> MQRCLARLFQAGVHTPHGSRYNAARMKNWPVQEVPQNFNFTNEQRFKAKAVPRDTGKIPRDFLLSVLYRNQPCEVASLWEHCLHDPQIVLDSKRHLREVLQQARAEGFVSFEKDAVTDRWVCHLTRERFEEVRALVGARAEAQDLYSGLRGASATETSAYSESFREMNEDTKREHFRLLSEQVADTTTHLRKFQ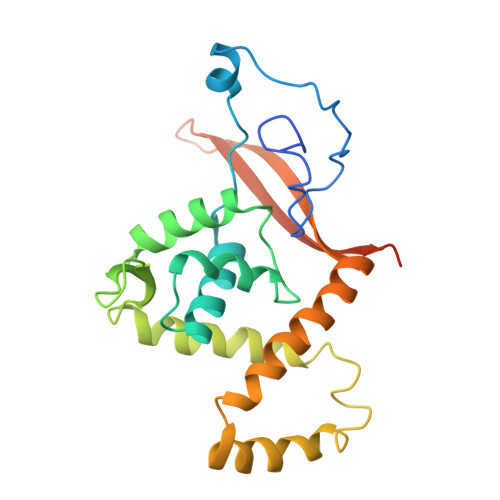RMEMDYLPYTDLNGKVNFMWWYEMSDTRDATALPEAAAEGSPKLSE>[2x]GGADQKGPVFLKEPTNRIDFSNSTGAEIECKASGNPMPEIIWIRSDGTAVGDVPGLRQISSDGKLVFPPFRAEDYRQEVHAQVYACLARNQFGSIISRDVHVRAVVQQFYESEVNNEYVIRGNAAVLKCSIPSFVADFVQVVSWQDEEGQLYGSLGDQQGTDGKYLVLPSGELHIREVGPEDGYKSYQCRTKHRLTGETRLSATKGR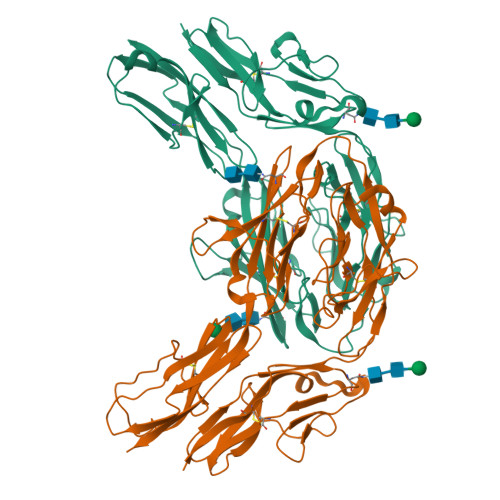LVITEPVGSVSPQLSGNGNQEHITLTRVPKMGSVTLMCPAQAYPVPFFRWYKFIEGTTRKQAVVLNDRVKQVSGTLIIKDAVVEDSGKYLCVVNNSVGGESVETVLTVTAPLSAKIDPPTQTVDFGRPAVFTCQYTGNPIKTVSWMKDGKAIGHSEPVLRIESVKKEDKGMYQCFVRNDQESAEASAELKLGG SOX proteins are a family of transcription factors (TFs) that play critical functions in sex determination, neurogenesis, and chondrocyte differentiation, as well as cardiac, vascular, and lymphatic development. There are 20 SOX family members in humans, each sharing a 79-residue L-shaped high mobility group (HMG)-box domain that is responsible for DNA binding. The L-shaped HMG-box comprises three α-helices: α1 and α2 that form one arm of the L (major wing), and α3 that forms the other arm of the L (minor wing). Here, we show that all SOX family members, except group H, interact with RNA.

Due to its inability to bind RNA, we sought to characterise the structure of the SOX30 HMG-box domain. Crystals formed in 0.1 M sodium acetate, 2 M ammonium sulphate, pH 4.6, and diffracted to 1.4 Å resolution. The crystal structure revealed that the SOX30 HMG-box domain contains the typical features of an HMG-box, including three α-helices and two disordered regions towards the N- and C-termini. Superimposing our SOX30 HMG-box domain structure on other available SOX protein HMG-box domain structures (alone and DNA-bound) demonstrated a very similar secondary structure between SOX family members, with a low RMSD. The C-terminal end of the SOX30 structure is seen to be orientated in a different direction to the other SOX structures. However, this is due to differences in crystal packing, with the SOX30 molecule within the asymmetric unit sandwiched between two adjacent SOX30 molecules, forming crystal contacts that stabilise the C-terminal end in this conformation. The seven amino acids at the C-terminal end of the HMG-box that we identified as critical for RNA binding (407-QPRPGKR-413; 73–79 HMG-box numbering) are not visible in the SOX30 structure. Structurally, the HMG-box domain of SOX30 retained all of the key features of other SOX proteins, with no obvious structural differences that would indicate why SOX30 does not bind RNA. Conversely, SOX30 has the sequence RPGKR, and thus has lost 40% of its positive charge within this cluster, which may contribute to the loss of RNA binding ability. Conversely, SOX30, which shows no RNA binding, features the sequence 70-WVYQPRP-76.

> SGHVKRPMNAFMVWARIHRPALAKANPAANNAEISVQLGLEWNKLSEEQKKPYYDEAQKIKEKHREEFPGWVYQPRPGKRKRFPLSVSNV> SNAMAEPTAPSDRSDPAGARTLVLMRHAAAGSAVRDHDRPLTPDGVRAATAAGQWLRGHLPAVDVVVCSTAARTRQTLAATGISAQVRYRDELYGGGVDEILAEVAAVPADASTVLVVGHAPTIPATGWELVRQSLLNRDADPSSGAGDELRHFAAGTFAVLSTTGAWADLAQAGAELQLV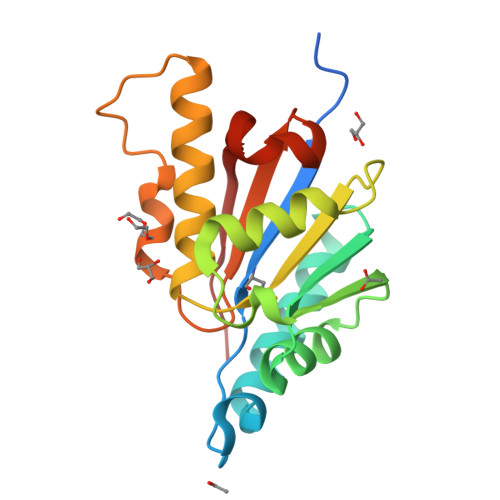QHPVA>[7x]MHHHHHHGTQQEALGMVETKGLTAAIEAADAMVASANVMLVGYEKIGCGLVTVIVRG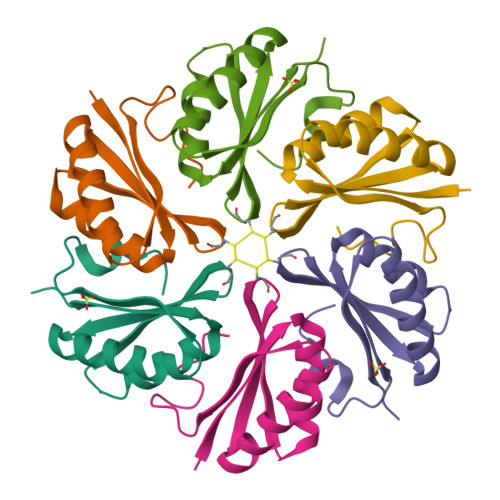DVGAVKAATDAGAAAARNVGEVKAVHVIPRPHTDVEKILPKGISQ>MQKYALHAYPVMALMVATLTGCAWIPAKPLVQGATTAQPIPGPVPVANGSIFQSAQPINYGYQPLFEDRRPRNIGDTLTIVLQENVSASKSSSANASRDGKTSFGFDTVPRYLQGLFGNSRADMEASGGNSFNGKGGANASNTFSGTLTVTVDQVLANGNLHVVGEKQIAINQGTEFIRFSGVVNPRTISGSNSVPSTQVADARIEYVGNGYINEAQNMGWLQRFFLNLSPM[26x];>MFKALAGIVLALVATLAHAERIRDLTSVQGVRENSLIGYGLVVGLDGTGDQTTQTPFTTQTLNNMLSQLGITVPTGTNMQLKNVAAVMVTASYPPFARQGQTIDVVVSSMGNAKSLRGGTLLMTPLKGVDSQVYALAQGNILVGGAGASAGGSSVQVNQLNGGRITNGAIIERELPTQFGAGNTINLQLNDEDFTMAQQITDAINRARGYGSATALDARTVQVRVPSGNSSQVRFLADIQNMEVNVTPQDAKVVINSRTGSVVMNREVTLDSCAVAQGNLSVTVNRQLNVNQPNTPFGGGQTVVTPQTQIDLRQSGGSLQSVRSSANLNSVVRALNALGATPMDLMSILQSMQSAGCLRAKLEII[26x]

The LP ring is a bushing supporting the distal rod for its rapid and stable rotation without much friction and is composed of a lipoprotein, FlgH, and a periplasmic protein, FlgI. The L and P rings are embedded within the outer membrane and the peptidoglycan (PG) layer, respectively. The P ring tightly associates with the PG layer, allowing the LP ring to act as a molecular bushing. Because the LP ring is required for efficient transport of hook and filament proteins into the culture media, it also functions as a secretion-like pore-forming annulus in addition to that as a molecular bushing.

Here we report the LP ring structure at 3.5 Å resolution, showing 26-fold rotational symmetry and intricate intersubunit interactions of each FlgH subunit with six FlgH partners that explains the structural stability. The inner and outer diameters of the LP ring are 135 Å and 260 Å, respectively, and its height is 145 Å. The L ring adopts a three-layer structure composed of two β-barrel layers and the outermost layer with an extended chain. The anti-parallel β strands of the inner and middle layer domains are crossing nearly perpendicular to each other, forming a hydrophobic core with conserved residues, and 26 copies of them form two layers of cylindrical β sheets in the inner and middle layers, respectively. The atomic model of FlgI contains residues 1–125, 138–263 and 296–346, which cover 87% of the entire FlgI sequence. It is composed of three domains, which we named FlgI-IRU (upper inner ring), FlgI-IRL (lower inner ring) and FlgI-OR (outer ring). The C-terminal half of the outer layer chain of a FlgH subunit (H0) lies at the bottom of the L ring and interacts with three FlgI subunits (I0, I±1) through its interactions with the hydrophobic inner and outer pockets of the P ring. Asp-78, Asp-86 and Glu-104 of FlgH form a negative charge belt, and Lys-69 and Lys-114 of FlgH form a positive charge belt, suggesting that both repulsive and attractive force keep the negatively charged rod rotating at the center of the L ring. We also found that Lys-63 and Lys-95, which are relatively well conserved among FlgI homologs, form a positive belt on the inner surface of the P ring and these residues are in very close proximity to a negative charge cluster on the rod outer surface, raising a plausible hypothesis that these two lysine residues are critical for P ring assembly around the rod. We therefore suggest that Lys-63 and Lys-95 of FlgI are essential for the initial binding of FlgI to the rod surface to form the P ring tightly attached to the rod and that some conformational changes occur in the P ring upon binding of FlgH for L ring assembly to make the completed LP ring free from the rod for its free, high-speed rotation within the LP ring as a bushing.> MANPLAGKPFYV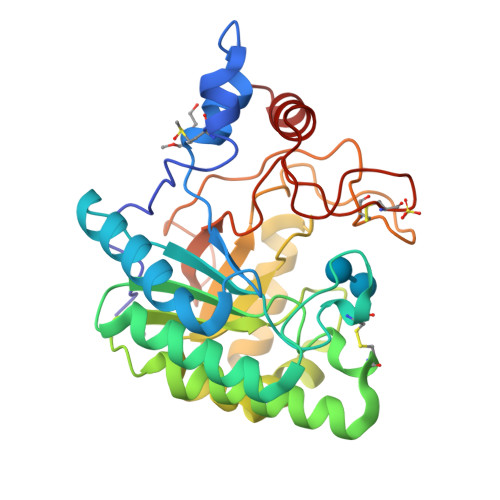DPASAAMVAARNANPPNAELTSVANTPQSYWLDQAFPPATVGGTVARYTGAAQAAGAMPVLTLYGIPHRDCGSYASGGFATGTDYRGWIDAVASGLGSSPATIIVEPDALAMADCLSPDQRQERFDLVRYAVDTLTRDPAAAVYVDAGHSRWLSAEAMAARLNDVGVGRARGFSLNVSNFYTTDEEIGYGEAISGLTNGSHYVIDTSRNGAGPAPDAPLNWCNPSGRALGAPPTTATAGAHADAYLWIKRPGESDGTCGRGEPQAGRFVSQYAIDLAHNAGQ(2-SULFANYL-3-PHENYLPROPANOYL)-PHE-TYR 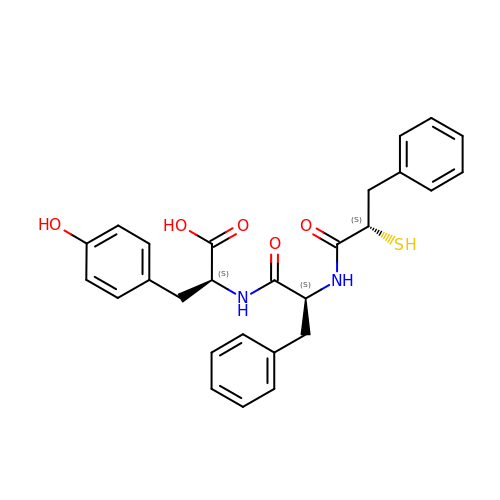| C27 H28 N2 O5 S | GIVBBFGMRNXKPE-HJOGWXRNSA-N> MHHHHHHTSVMSHEFQLATAETWPNPWPMYRALRDHDPVHHVVPPQRPEYDYYVLSRHADVWSAARDHQTFSSAQGLTVNYGELEMIGLHDTPPMVMQDPPVHTEFRKLVSRGFTPRQVETVEPTVRKFVVERLEKLRANGGGDIVTELFKPLPSMVVAHYLGVPEEDWTQFDGWTQAIVAANAVDGATTGALDAVGSMMAYFTGLIERRRTEPADDAISHLVAAGVGADGDTAGTLSILAFTFTMVTGGNDTV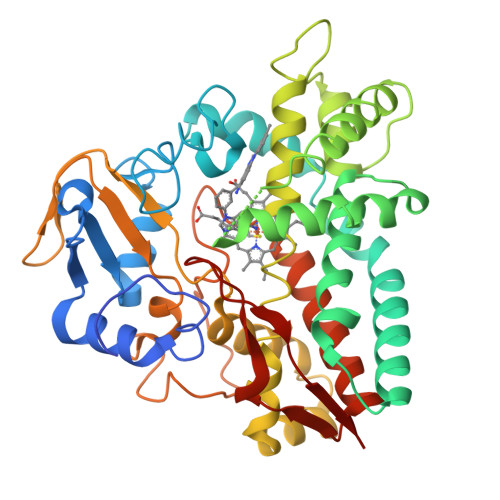TGMLGGSMPLLHRRPDQRRLLLDDPEGIPDAVEELLRLTSPVQGLARTTTRDVTIGDTTIPAGRRVLLLYGSANRDERQYGPDAAELDVTRCPRNILTFSHGAHHCLGAAAARMQCRVALTELLARCPDFEVAESRIVWSGGSYVRRPLSVPFRVTSSR> MFENITAAPADPILGLADLFRADERPGKINLGIGLYYDETGKIPVLTSVKKAEQYL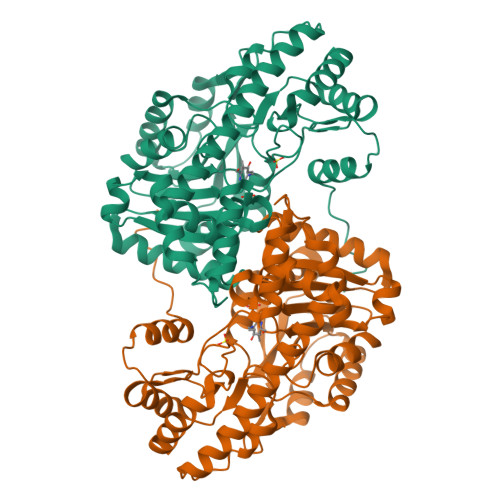LENETTKLYLGIDGIPEFGRCTQELLFGKGSALINDKRARTAQTPGGSGALRVAADFLAKNTSVKRVWVSNPSWPNHKSVFNSAGLEVREYAYYDAENHTLDFDALINSLNEAQAGDVVLFHGCCHNPTGIDPTLEQWQTLAQLSVEKGWLPLFDFAYQGFARGLEEDAEGLRAFAAMHKELIVASSYSKNFGLYNERVGACTLVAADSETVDRAFSQMKAAIRDNYSSPPAHGASVVATILSNDALRAIWEQELTDMRQRIQRMRQLFVNTLQEKGANRDFSFIIKQNGMFSFSGLTKEQVLRLREEFGVYAVASGRVNVAGMTPDNMAPLCEAIVAVL> 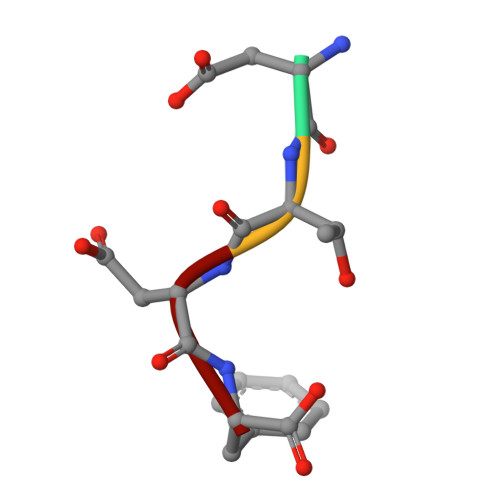DTDF>MGHHHHHQHMSTKQKLVGDVFSSVANRYDLMNDVMSLGIHRLWKDHFINKLDAGKRPNSTTPLNFIDVAGGSGDIAFGLLDHAESKFG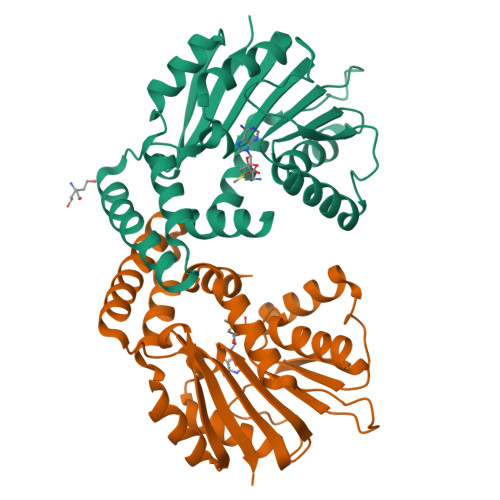DTESTMDIVDINPDMLKEGEKRAMEQGKYFKDPRVRFLVSNGEKLEEIDSDSKDIYTVSFGIRNFTDIQKGLNTAYRVLKPGGIFYCLEFSKIENPLMDFAYQQWAKVLPVMGSMIANDYDSYQYLVESIERFPDQETFKSMIEKAGFKSAGYESLTFGICAIHWGIKV[4x]> GAMASD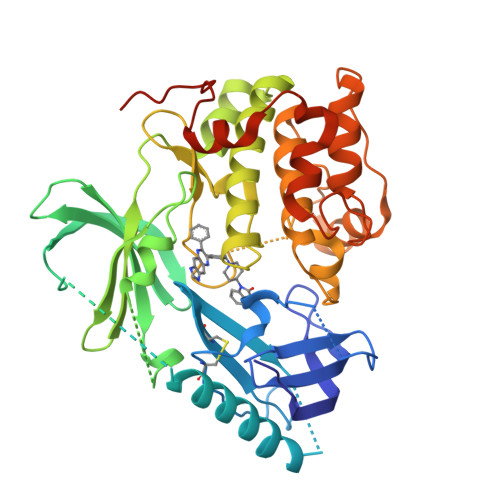VAIVKEGWLHKRGEYIKTWRPRYFLLKNDGTFIGYKERPQDVDQREAPLNNFSVAQCQLMKTERPRPNTFIIRCLQWTTVIERTFHVETPEEREEWTTAIQTVADGLKKQEEEEMDFRSGSPSDNSGAEEMEVSLAKPKHRVTMNEFEYLKLLGKGTFGKVILVKEKATGRYYAMKILKKEVIVAKDEVAHTLTENRVLQNSRHPFLTALKYSFQTHDRLCFVMEYANGGELFFHLSRERVFSEDRARFYGAEIVSALDYLHSEKNVVYRDLKLENLMLDKDGHIKITDFGLCKEGIKDGATMKTFCGTPEYLAPEVLEDNDYGRAVDWWGLGVVMYEMMCGRLPFYNQDHEKLFELILMEEIRFPRTLGPEAKSLLSGLLKKDPKQRLGGGSEDAKEIMQHRFFAGIVWQHVYEKKLSPPFKPQVTSETDTRYFDEEFT>MENFEIWVEKYRPRTLDEVVGQDEVIQRLKGYVERKNIPHLLFSGPPGTGKTATAIALARDLFGENWRDNFIEMNASDERGIDVVRHKIKEFARTAPIGGAPFKIIFLDEADALTADAQAALRRTMEMYSKSCRFILSCNYVSRIIEPIQSRCAVFRFKPVPKEAMKKRLLEICEKEGVKITEDGLEALIYISGGDFRKAINALQGAAAIGEVVDADTIYQITATARPEEMTELIQTALKGNFMEARELLDRLMVEYGMSGEDIVAQLFREIISMPIKDSLKVQLIDKLGEVDFR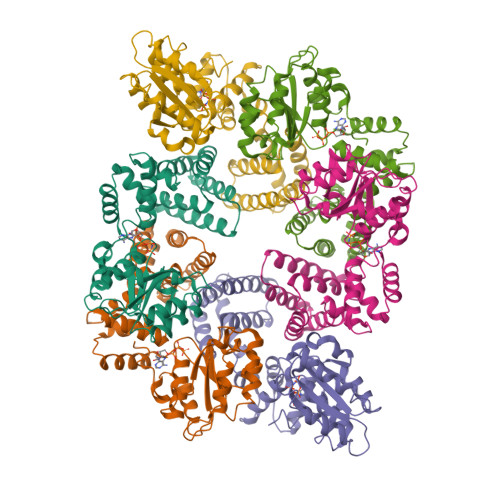LTEGANERIQLDAYLAYLSTLAKK[3x]> NANRSKEWKNAANTLLFGLDESVDPCEDFYGFTCNKFIERIDLDELGRGRFTTFSQAQLEVNSDIVKALEKVDVNDEKFSQTE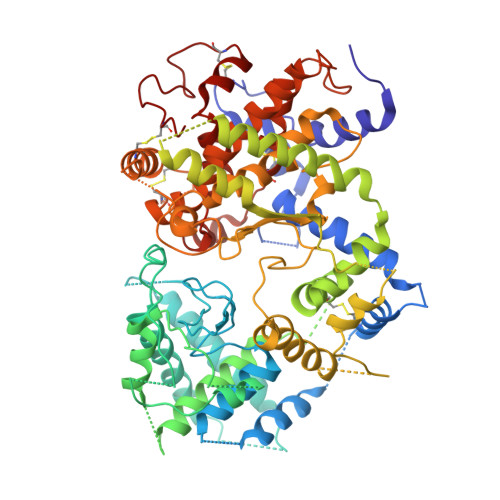RITKAAFQSCVEYTLKDDRKASVNELLQYISERFGGIPFLGQRVKGGCELYREMGRIEQQRALPTFMYTWVNVDHKNVSRNSYYISQPTLPMPREFYVLPQFAPELDARTKAIENVMKAFASDILKDPSKYDKMIKTAAREVTQIEQKIAMASWPDDELRNHEQQYNPYELFAPSEGKIALQDAFPNIRFGKYIAGLMETATGGVPVSPVFIGDVIVTNPAYMGFLNTLFRQTNIQMNQYPFVNYIIVHMLFEDAEHLGDKYLRIAKDADYVTYAQRKGVGITRSGRKYSRVFDERTDARMKCVDTITTYMPYGTGYVYVNSREDRDQVVEDVKQQTELIMKTFLKKMLSTLSWMQGESYRRAEKKINEMHRNYGWPKKLFGDFKNFDTIDAYHRDDYYSILEAYNNKTDKSTAFYTILNILRRGYENRESFRRKNETADRTNFLESPASVNAWYAPELNSLTLPFGILTSPHYDLQFPKAFNFAGSGTVGGHELVHGFDDEGVQFDYDGSLADCSVYECGWLEQKGKNGFKDMAQCVVTQYNAQCCPAKEGNVHCANGAHTQGENIADLGGLQASYNAYKEYIKMKGAEEMRLPGLEKFTPNQIFWISYGYSWCAKETQSSLVKRLLTNPHSPNSCRVNQVLQDIPSFAKDFQCALGQKMYPPAEQRCKVW> HRELGS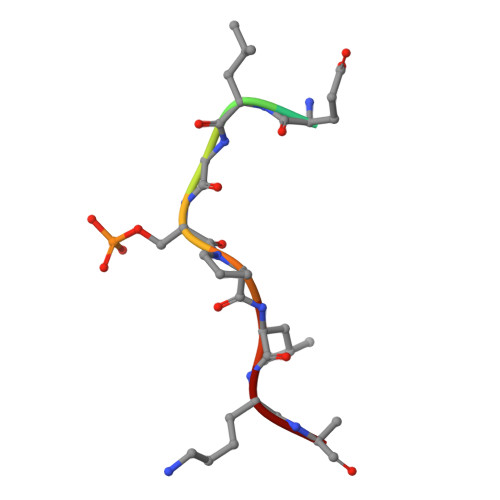PLKK5'-O-[(S)-hydroxy{[(S)-hydroxy{[(R)-hydroxy(phosphonooxy)phosphoryl]oxy}phosphoryl]oxy}phosphoryl]guanosine 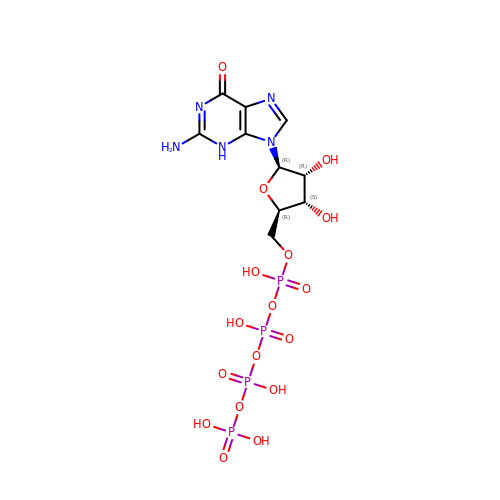| C10 H17 N5 O17 P4 | KDFXXNGTULMGMF-UUOKFMHZSA-N3-chloranyl-2,6-bis(fluoranyl)phenol | C6 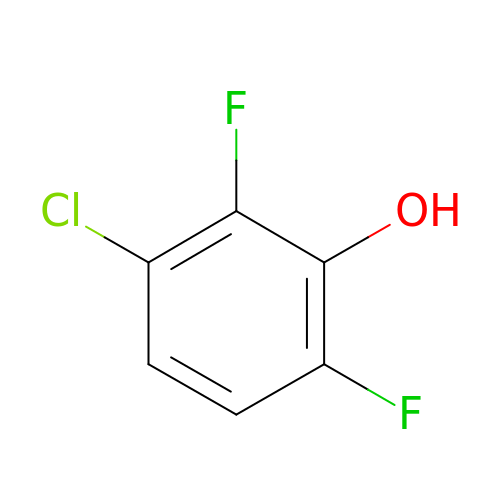H3 Cl F2 O | CCLYWHXHYLQWQK-UHFFFAOYSA-N> ADFEVHMLNKGKDGAMVF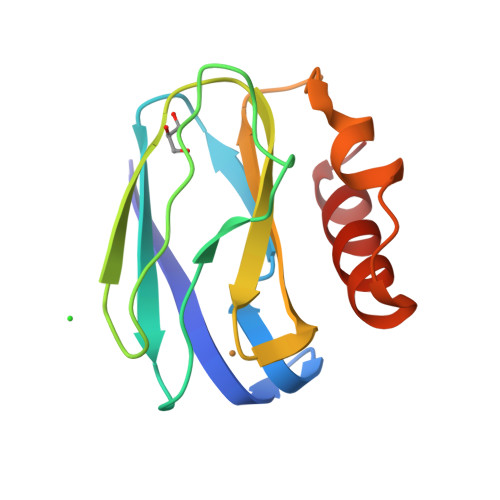EPASLKVAPGDTVTFIPTDKGHNVETIKGMIPDGAEAFKSKINENYKVTFTAPGVYGVKCTPHPFMVGVVQVGDAPANLEAVKGAKNPKKAQERLDAALAALGN>[2x]GAGSTAGKVIKCKAAV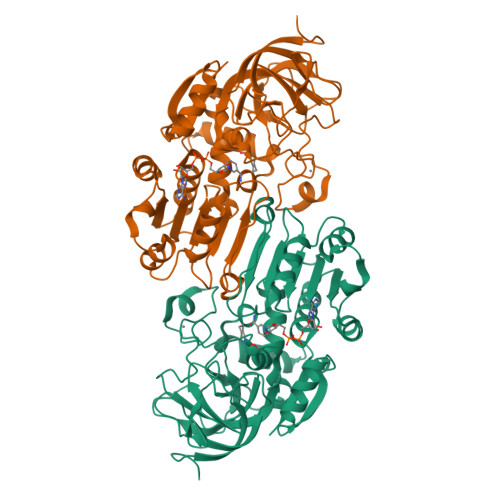LWEEKKPFSIEEVEVAPPKAHEVRIKMVATGICRSDDHVVSGTLVTPLPVIAGHEAAGIVESIGEGVTTVRPGDKVIPLFTPQCGKCRVCKHPEGNFCLKNDLSMPRGTMQDGTSRFTCRGKPIHHFLGTSTFSQYTVVDEISVAKIDAASPLEKVCLIGCGFSTGYGSAVKVAKVTQGSTCAVFGLGGVGLSVIMGCKAAGAARIIGVDINKDKFAKAKEVGATECVNPQDYKKPIQEVLTEMSNGGVDFSFEVIGRLDTMVTALSCCQEAYGVSVIVGVPPDSQNLSMNPMLLLSGRTWKGAIFGGFKSKDSVPKLVADFMAKKFALDPLITHVLPFEKINEGFDLLRSGESIRTILTF(1S,3Z)-3-[(2E)-2-[(1R,3AR,7AS)-7A-METHYL-1-[(2R)-6-METHYLHEPTAN-2-YL]-2,3,3A,5,6,7-HEXAHYDRO-1H-INDEN-4-YLIDENE]ETHYLIDENE]-4-METHYLIDENE-CYCLOHEXAN-1-OL 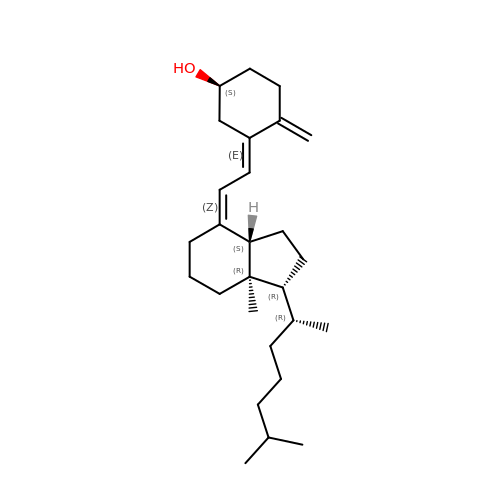| C27 H44 O | QYSXJUFSXHHAJI-RWDMXNMGSA-N> P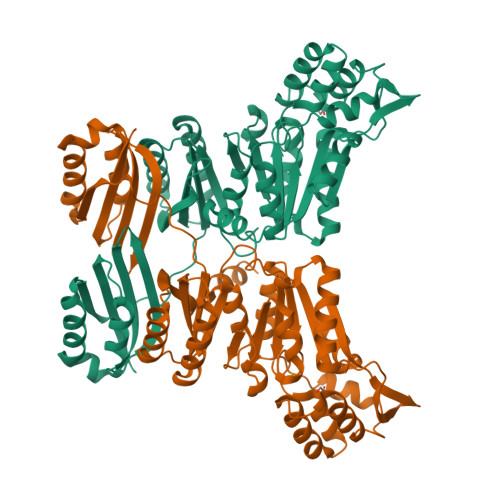KVSVLITVTGVDQPGVTATLFEVLSRHGVELLNVEQVVIRHRLTLGVLVCCPADVADGPALRHDVEAAIRKVGLDVSIERSDDVPIIREPSTHTIFVLGRPITAAAFGAVAREVAALGVNIDLIRGVSDYPVIGLELRVSVPPGADGALRTALNRVSSEEHVDVAVEDYTLERRAKRLIVFDVDSTLVQGEVIEMLAAKAGAEGQVAAITDAAMRGELDFAQSLQQRVATLAGLPATVIDEVAGQLELMPGARTTLRTLRRLGYACGVVSGGFRRIIEPLAEELMLDYVAANELEIVDGTLTGRVVGPIIDRAGKATALREFAQRAGVPMAQTVAVGGGANDIDMLAAAGLGIAFNAKPALREVADASLSHPYLDTVLFLLGVTRGEIEAADAID> SDKPVAHVVANHQVEEQLEWLSQRANALLANGMDLKDNQLVVP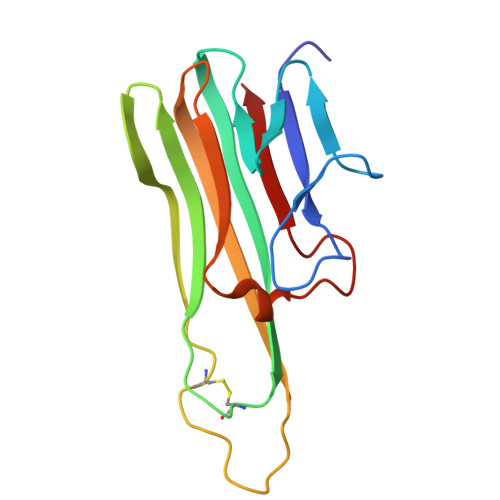ADGLYLVYSQVLFKGQGCPDYVLLTHTVSRFAISYQEKVNLLSAVKSPCPKDTPEGAELKPWYEPIYLGGVFQLEKGDQLSAEVNLPKYLDFAESGQVYFGVIAL>[2x]MEDFYTYKFSLWKIRIIKRFFPTVKGNLSSRQEVEDLCQKKGKIRLLVWGSTLENERVNFNKSVEVYRLEDGFIRSIGLGIRLSIPISLVADPIGIYYDATKPSYLEEILLARKFDNVILERAQRVIELLRRYKITKYNISTDK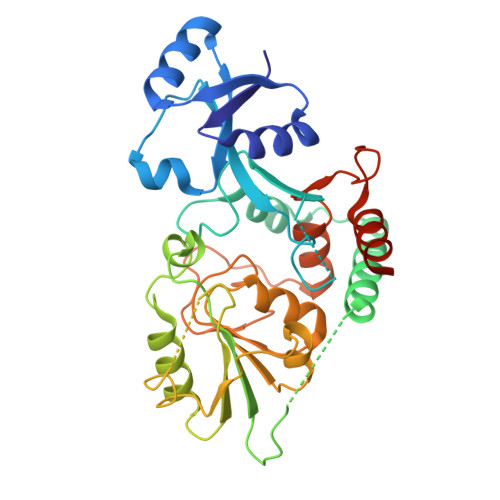KWRPPRTDKKIIVVPGQVESDASIKFGSPYIKTNLELLKSVREHNPNAYIVYKPHPDVVGGYRKGSYKPGELLKFCDEICVNSSSYDIISYADEVHVLTSLFGFEALIAGKPVTCYGHPFYAGYGLTTDIYPHPRRNIKLSLQELVAGALLLYPMYVSLIDGNRISAEEAIFELVNLKKNLPHHHHHH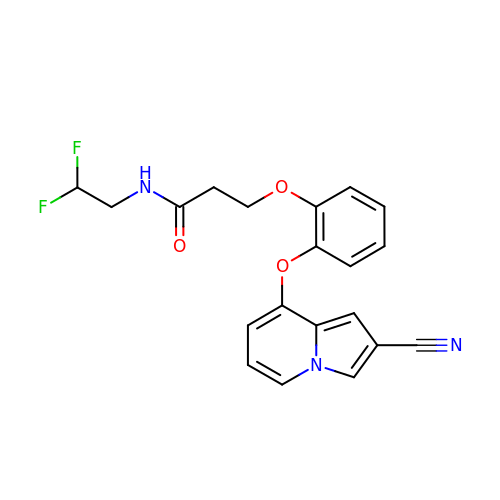3-(2-{[(4R)-2-cyanoindolizin-8-yl]oxy}phenoxy)-N-(2,2-difluoroethyl)propanamide | C20 H17 F2 N3 O3 | PTNLADVCXMBZFS-UHFFFAOYSA-N> LPTSNPAQELEARQLGRTTRDDLINGNSASCADVIFIYARGSTETGNLGTLGPSIASNLESAFGKDGVWIQGVGGAYRATLGDNALPRGTSSAAIREMLGLFQQANTKCPDATLIAGGYSQGAALAAASIEDLDSAIRDKIAGTVLFGYTKNLQNRGRIPNYPADRTKVFCNTGDLVCTGSLIVA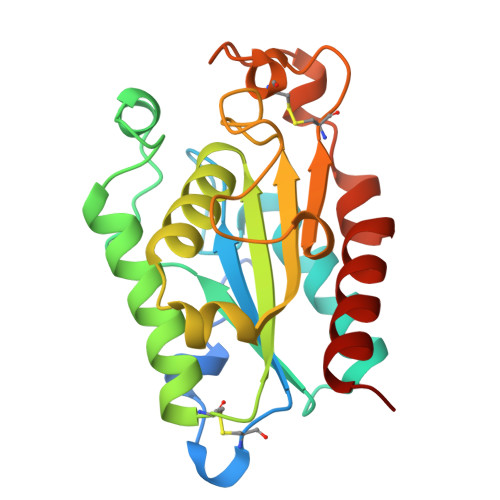APHLAYGPDAEGPAPEFLIEKVRAVRGSA> GAMDPEFMDAKARNCLLQHREALEKDIKTSYIMDHMISNGVLSVIEEEKVKSQATQYQRAAALIKMILNKDNCAYISFYNALLHEGYKDLAALLQSGLPLVSSSSGKDTDGGITSFVRTVLCEGGVPQRPVIFVTRKKLVHAIQQKLWKLNGEPGWVTIYGMAGCGKSVLAAEAVRDHSLLEGCFSGGVHWVSIGKQDKSGLLMKLQNLCMRLDQEESFSQRLPLNIEEAKDRLRVLMLRKHPRSLLILDDVWDPWVLKAFDNQCQILLTTSDKSVTDSVMGPKHVVPVESGLGREKGLEILSLFVNMKKEDLPAEAHSIIKECKGSPLVVSLIGALLRDFPNRWAYYLRQLQNKQFKRIRKSSSYDYEALDEAMSISVEMLREDIKDYYTDLSILQKDVKVPTKVLCVLWDLETEEVEDILQEFVNKSLLFCNRNGKSFCYYLHDLQVDFLTEKNRSQLQDLHRKMVTQFQRYYQPHTLSPDQEDCMYWYNFLAYHMASANMHKELCALMFSLDWIKAKTELVGPAHLIHEFVAYRHILDEKDCAVCENFQEFLSLNGHLLGRQPFPNIVQLGLCEPETSEVYRQAKLQAKQEGDTGRLYLEWINKKTIKNLSRLVVRPHTDAVYHACFSQDGQRIASCGADKTLQVFKAETGEKLLDIKAHEDEVLCCAFSSDDSYIATCSADKKVKIWDSATGKLVHTYDEHSEQVNCCHFTNKSNHLLLATGSNDFFLKLWDLNQKECRNTMFGHTNSVNHCRFSPDDELLASCSADGTLRLWDVRSANERKSINVKRFFLSSEDPPEDVEVIVKCCSWSADGDKIIVAAKNKVLLFDIHTSGLLAEIHTGHHSTIQYCDFSPYDHLAVIALSQYCVELWNIDSRLKVADCRGHLSWVHGVMFSPDGSSFLTASDDQTIRVWETKKVCKNSAIVLKQEIDVVFQENETMVLAVDNIRGLQLIAGKTGQIDYLPEAQVSCCCLSPHLEYVAFGDEDGAIKIIELPNNRVFSSGVGHKKAVRHIQFTADGKTLISSSEDSVIQVWNWQTGDYVFLQAHQETVKDFRLLQDSRLLSWSFDGTVKVWNVITGRIERDFTCHQGTVLSCAISSDATKFSSTSADKTAKIWSFDLLSPLHELKGHNGCVRCSAFSLDGILLATGDDNGEIRIWNVSDGQLLHSCAPISVEEGTATHGGWVTDVCFSPDSKTLVSAGGYLK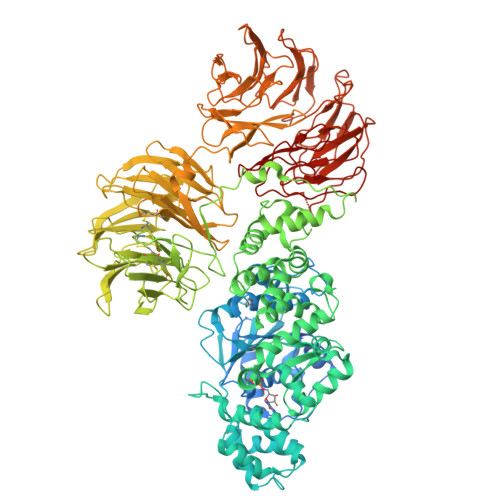WWNVATGDSSQTFYTNGTNLKKIHVSPDFRTYVTVDNLGILYILQVLE>[4x]SATTIQKELENIVVKERQNKKDTILMGLKVEVPWNYCDWASISFYDVRLESGILDMESIAVKYMTGCDIPPAVTLGITNKDQEA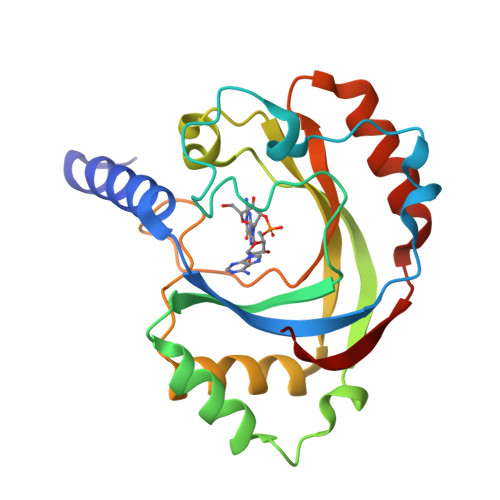NFQRFKELTRNIDLTSLSFTCKEVICFPQSRASKELGANGRAVVMKLEASDDVKALRNVLFNVVPTPRDIFGPVLSDPVWCPHVTIGYVRADDEDNKNSFIELAEAFRGSKIKVIGWCE N-[(2R,3S,4R,5R,6R)-4,5-dihydroxy-2,6-bis(hydroxymethyl)piperidin-3-yl]acetamide | C9 H18 N2 O5 | 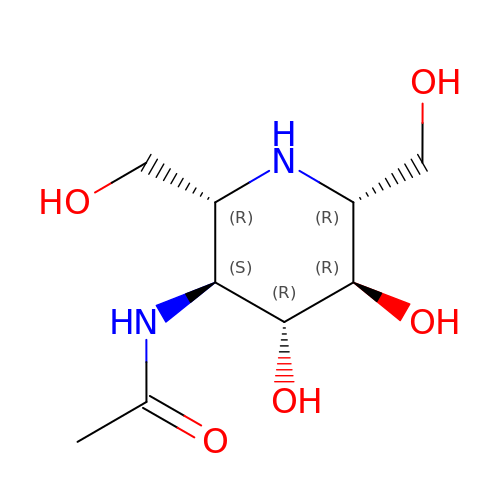GYKHMAHAJKZLAT-KVEIKIFDSA-N>[2x]GRKERERLEEK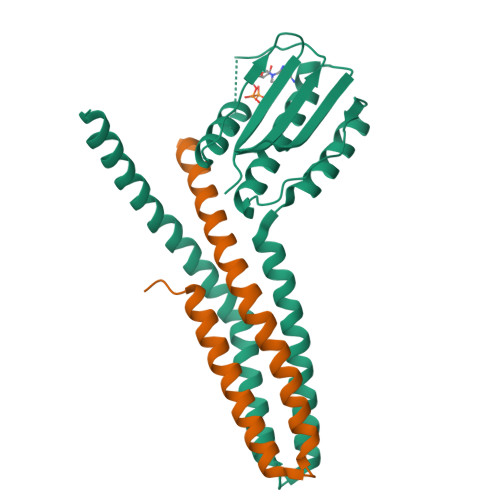LEDANERIAELVKLEERQRIARDLEDTLGQKLSLIGLKSDLARKLIYKDPEQAARELKSVQQTARTSLNEVRKIVSSMKGIRLKDELINIKQILEAADIMFIYEEEKWPENISLLNENILSMCLKEAVTNVVKHSQAKTCRVDIQQLWKEVVITVSDDGTFKGEENSFSKGHGLLGMRERLEFANGSLHIDTENGTKLTMAIPNNSK3-methyl-N-{[(3S)-oxolan-3-yl]methyl}-1,2-oxazole-5-carboxamide 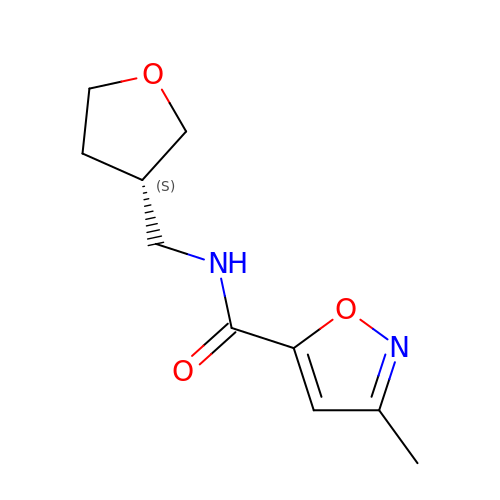| C10 H14 N2 O3 | VMYFKAZPRAZUQC-QMMMGPOBSA-N> MAHHHHHHMKTSTIVFGGFFITDNGERIQIPILENPNIKEINNFFSVSNFEKKAGVLVF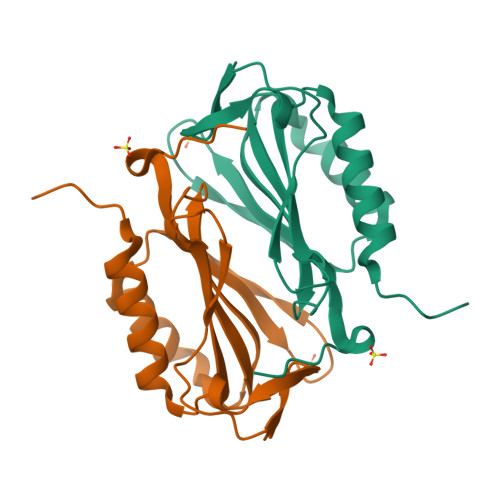RIIPEPEFGNTELTIYFEKGYYLPIIQTILEDGDIEVKNLKTENYSGNTMEILGDVYPIEHISKNISIIQDIISEFIMKNKPITIMI>MKKHTGYVGLKNQGATCYMNSLLQTLFFTNQLRKAVYMMPTEGDDSSKSVPLALQRVFYE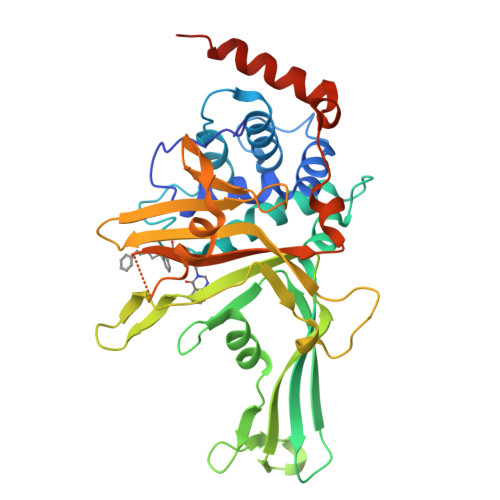LQHSDKPVGTKKLTKSFGWETLDSFMQHDVQELCRVLLDNVENKMKGTCVEGTIPKLFRGKMVSYIQCKEVDYRSDRREDYYDIQLSIKGKKNIFESFVDYVAVEQLDGDNKYDAGEHGLQEAEKGVKFLTLPPVLHLQLMRFMYDPQTDQNIKINDRFEFPEQLPLDEFLQKTDPKDPANYILHAVLVHSGDNHGGHYVVYLNPKGDGKWCKFDDDVVSRCTKEEAIEHNYGGHDDDLSVRHCTNAYMLVYIRESKLSEVLQAVTDHDIPQQLVERLQEEKRIEAQKRKERQEHHHHHH[2x]> MKKLFLVFWWHMHQPLYREPYTGEYLLPWTFFHAVKDYYDMPAYLKDFEIKLNFNLTPVLIDQIQEYAQGKAKDVFLEAIRKDPDDLEKEEVEKLIEFTKLNYEKPIYRFERIRELMNKEKLNREELLDLQTLNLLAWCGRTLRKDLKDLLNKGRNYTQEEKEYVLNKY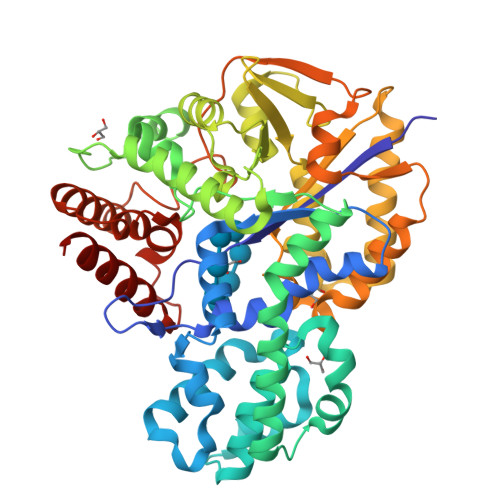FEIIKKTLSIYREIKEEGKGSVSTSPYYHPLIPILLNPNCVYETTPNVKIPDFAVSFREDASKHVELAKEKYFEIFGEHPVYMWPPEASVSNEALELYYEKGINMLATDEVILKNSVERASPYLRYYFRELISVFFRDKTLSDLIGFSYHAWNAEDAVRDFIGRLKKIHESVDFQPVVFVVLNGENCWEYYEENGIPFLEKLYSTLEKEEWIETLTLEEAMRKEDVKTEVIESVKAGTWFDGNFLKWIGNKEKNEYWKILIEAKKKAKNDYILVAEGSDWFWWQGEEKAPFVEVFDKLFRSFVRRAQE>[4x]ADDAKPRVKVPSSAKAGETVTVKALISHKME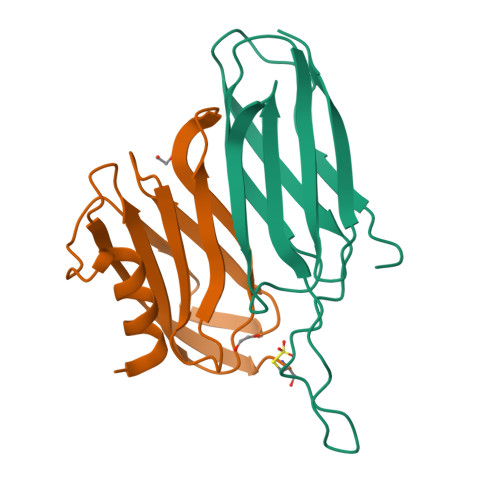SGQRKDADGKLIPRSIINRFTCELNGVNVVDVAIDPAVSTNPYFEFDAKVDAAGEFKFTWYDDDGSVYEDVKPIAV;>[4x]MRGSHHHHHHGSSTVDELTAAFTGGAATGEGGLTLTAPEIAENGNTVPIEVKAPGAVAIMLLAAGNPEPAVATFNFGPAAADQRAATRIRLAQTQDVIALAKMADGSVVKAQTTVKVTIGGCGG> KWPEPVFGRLVSPGFPEKYGNHQDRSWTLTAPPGFRLRLYFTHFNLELSYRCEYDFVKLTSGTKVL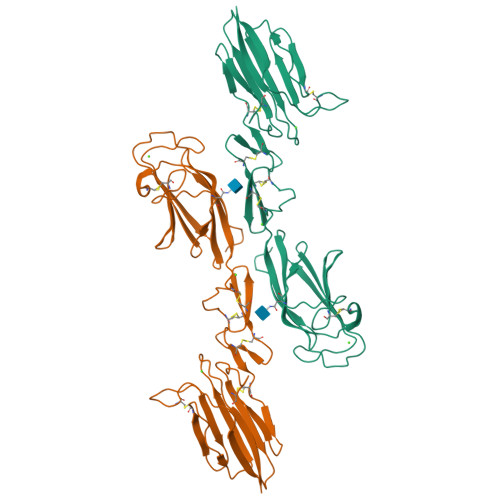ATLCGQESTDTERAPGNDTFYSLGPSLKVTFHSDYSNEKPFTGFEAFYAAEDVDECRTSLGDSVPCDHYCHNYLGGYYCSCRVGYILHQNKHTCSALCSGQVFTGRSGFLSSPEYPQPYPKLSSCAYNIRLEEGFSITLDFVESFDVEMHPEAQCPYDSLKIQTDKREYGPFCGKTLPPRIETDSNKVTITFTTDESGNHTGWKIHYTSTA> TAPSQVLKIRRPDDWHLHLRDGDMLKTVVPYTSEIYGRAIVMPNLAPPVTTVEAAVAYRQRILDAVPAGHDFTPLMTCYLTDSLDPNELERGFNEGVFTAAKLYPA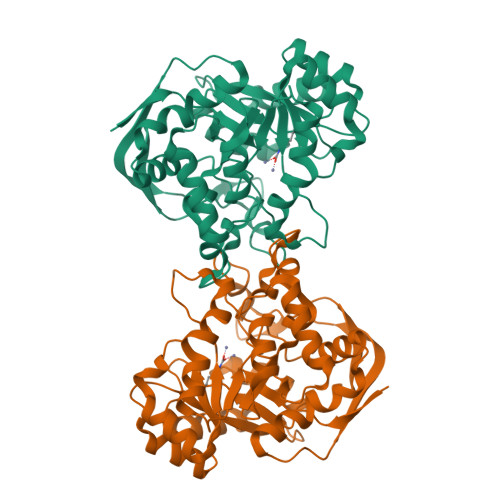TSVDAIMPVLERMEKIGMPLLVHGEVTHADIDIFDREARFIESVMEPLRQRLTALKVVFEHITTKDAADYVRDGNERLAATITPQHLMFNRNHMLVGGVRPHLYCLPILKRNIHQQALRELVASGFNRVFLGTDSAPHARHRKESSCGCAGCFNAPTALGSYATVFEEMNALQHFEAFCSVNGPQFYGLPVNDTFIELVREEQQVAESIALTDDTLVPFLAGETVRWSVKQ>[6x]HHHHHHMSMRDAVICEPVRTPIGRYGGMFRSLTAVDLGVTALKGLLERTGIAADQVEDVILGHCYPNSEAPAIGRVVALDAGLPITVPGMQVDRRCGSGLQAVIQACLQVRSGDHDLVVAGGAESMSNVAFYSTDMRWGGARTGVQIHDGLARGRTTAGGKFHPVPGGMLETAENLRREYHISRTEQDELAVRSHQRAVAAQSEGVLAEEII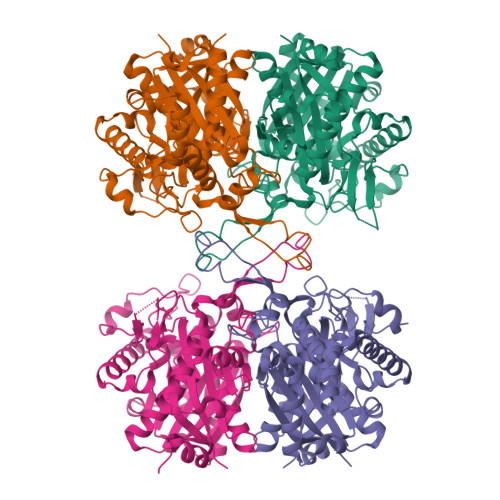PVPVRTRDGEETISVDEHPRADTTVEALAKLKPVLLKQDPEATVTAGNSSGQNDAASMCIVTTPEKAAELGLKPLVRLVSWGSAGVAPDLMGIGPVPATEVALAKAGLTLADIDLIELNEAFAAQALAVMREWKFGEADHERTNVRGSGISLGHPVGATGGRMLATLARELHRREARYGLETMCIGGGQGLAAVFERVQEG> MFPSPRAQGMGSARRPFNSRLTGGRKALGPGVTASSSPSALYSPVGRRVSASGARSTPSRVYLHPAASETVNYNVQLFGSSLPVKVMEALSNASADEPMAACIHEGGWAWLACNDRLIIWKISHSSSAKLMVCKELPLPLSDSEWSADLVDICAQTGDPAAAQSVALMAATPEGSSRYWPNILHEGTYIESYTEFGSSLCAFVTAVKGNSFILSSEKNQLVRLTPDASGKMNQRVLPQGQGMLSGIGRRVSTLFGILSPAVESTLCSVLWDKGDCFYTLTDSSINKWDLDDTSESQVLNWDMSRVLREYISDAIWGSESDYDDIKAGININYLSLNQNCDGLVILSAAWHPGDNPCQIYYTLVTVKDEGYNISDEITVEVTQFNPVFQARGMQLCQLVVPNFSSQACYLYTQEMIFACSTGTGRSTLPQEKIPFEAQGDNIVGAGSCEGWPVFFIRKSGMLTVVARETASVLPEHMEESLSSVSKSSRQAVVKDSRPDQIAHDDKTKHLKAAFLRYCRKDILGAQSMVDSLFSDSDMEPDDELDLAVNQISVDLIDDYPASDPRWAESVPEEAAGFSNTSLILLHQLEDKMKAHSFFVDFLHQVGLFSRLSTCQTKGMLVATRLLLSEHAEKLSAAIVLKNHHAKLPVLVNSAIQLALDKRMCTVPQNLTAADVYFREVSQMEIIFECLVDKEEADLESTSIDSVEWANIVV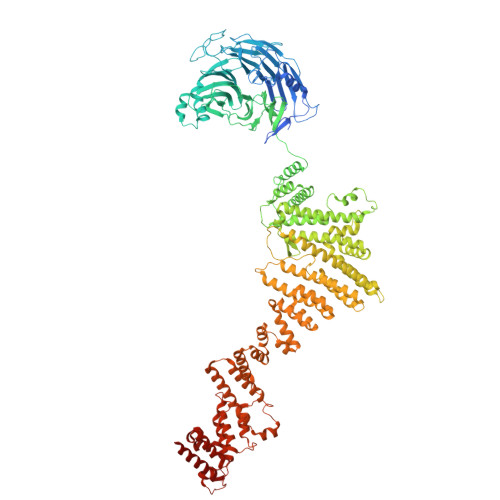NVNTILKDMLHVACQYRQSKNSLYKNESGIQEPEHVPWTASSGTAGIRSVVTRQHGIILKVYPQADSGLRTILIEQLAALLNYLLDDYVTQLKSIDKLANEERYNILEMEYAQKRSELLSPLLILGQYAWASNLAEKYCDFDILVQICEMTDNQSRLQRYMTLFAEQNFSDFLFRWYLEKGKRGKLLSQPASQHGQLAAFLQAHDHLSWLHELNSQEFEKAHRTLQTLANMETRYFCKKKTLLGLSKLAALASDFQEDVLQEKVEEIAEQEHFLLHQETLPKKLLEEKQLDLNAMPVLAPFQLIQLYVCEENKRANENDFMKALDLLEYIGDDSEVDVEELKLEILCKAIKRDEWSATDGKDDPIEATKDSIFVKVLQNLLNKGIELKGYLPKAETLLQSEELNSLKTNSYFEFSLKANYECYMKMQS> EDII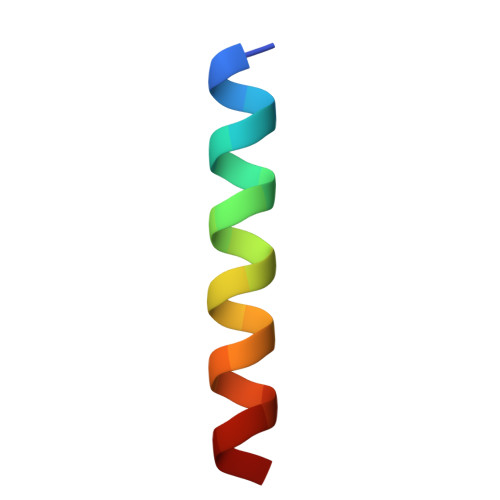RNIARHLAQWGDSMDRSW[[(2~{R},3~{S},4~{R},5~{R})-5-(6-aminopurin-9-yl)-4-oxidanyl-3-phosphonooxy-oxolan-2-yl]methoxy-oxidanyl-phosphoryl] [(3~{R})-4-[[3-[2-[(~{E})-2-[3,5-bis(oxidanyl)phenyl]-1-oxidanyl-ethenyl]sulfanylethylamino]-3-oxidanylidene-propyl]amino]-2,2-dimethyl-3-oxidanyl-4-oxidanylidene-butyl] hydrogen phosphate | C29 H42 N7 O19 P3 S | 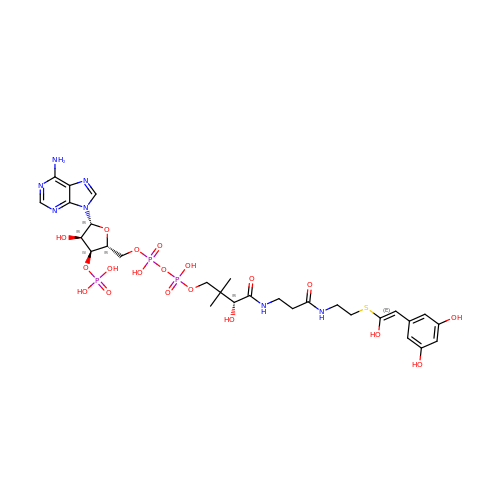LMMCTIXJVGWLEK-NUSWKBOXSA-N> MLSNSQGQSPPVPFPAPAPPPQPPTPALPHPPAQPPPPPPQQFPQFHVKSGLQIKKNAIIDDYKVTSQVLGLGINGKVLQIFNKRTQEKFALKMLQDCPKARREVELHWRASQCPHIVRIVDVYENLYAGRKCLLIVMECLDGGELFSRIQDRGDQAFTEREASEIMKSIGEAIQYLHSINIAHRDVKPENLLYTSKRPNAILKLTDFGFAKETTSHNSLTTPCYTPYYVAPEVLGPEKYDKSCDMWSLGVIMYILLCGYPPFYSNHGLAISPGM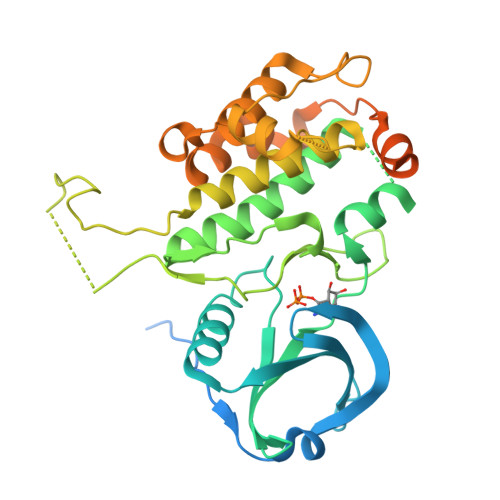KTRIRMGQYEFPNPEWSEVSEEVKMLIRNLLKTEPTQRMTITEFMNHPWIMQSTKVPQTPLHTSRVLKEDKERWEDVKEEMTSALATMRVDYEQIKIKKIEDASNPLLLKRRKKARALEAAALAH>TRDANGTWEMESNENFEGWMKALDIDFALRKIAVRLTLTLVIDQDGDNFKVKCTSTFWNYDVDFTVGVEFDEYTK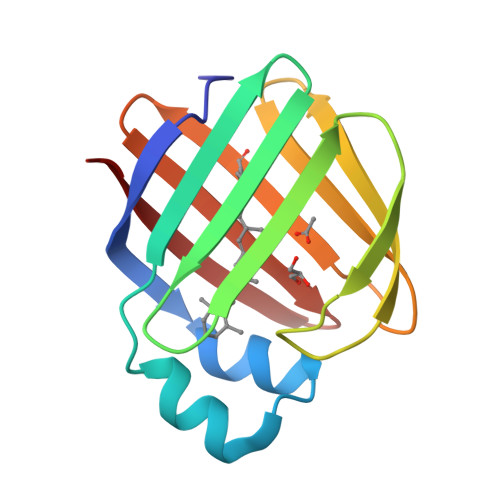SLDNRHVKALVTWEGDVLVCVQKGEKENRGWKKWIEGDKLYLELTCGDQVCRQVFKKK[2x]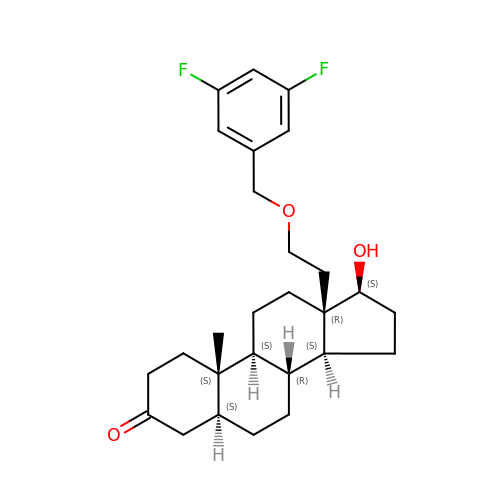(5S,8R,9S,10S,13R,14S,17S)-13-{2-[(3,5-DIFLUOROBENZYL)OXY]ETHYL}-17-HYDROXY-10-METHYLHEXADECAHYDRO-3H-CYCLOPENTA[A]PHENANTHREN-3-ONE | C27 H36 F2 O3 | AJODXHGZHBERGJ-JLYQOUBASA-N The type VI secretion system (T6SS) is a widespread protein export apparatus found in Gram-negative bacteria. T6SSs mediate bacterial antagonism by facilitating the injection of toxic effector proteins into competing bacterial cells in a contact-dependent manner. Here, we present the structures of the T6SS effector RhsA from Pseudomonas protegens and its cognate T6SS spike protein, VgrG1, at 3.3 Å resolution. The rhsA operon contains genes encoding its cognate VgrG spike and Eag chaperone proteins, both of which are required for the delivery of this effector into susceptible competitors.

To investigate how RhsA is mounted onto VgrG1 we set out to determine the structure of the secretion competent pre-firing complex (PFC) comprising VgrG1 in complex with full-length RhsA and EagR1. Unfortunately, this conformational heterogeneity prevented us from obtaining a high-resolution 3D reconstruction of the entire complex. Instead, we applied C3 symmetry during processing to determine the three-dimensional structure of P. protegens VgrG1. In applying this symmetry operator, the RhsA and EagR1 components of the complex, which do not adopt this symmetry, are averaged out during image processing. The cryo-EM map of VgrG1 reached a resolution of 3.3 Å and allowed us to build almost the complete atomic model of the protein comprising residues 8–643. As expected, given its high sequence homology, the structure of VgrG1 from P. protegens is nearly identical (71% sequence identity, 81% sequence similarity) to our previously determined VgrG1 structure from P. aeruginosa (r.m.s.d of 1.035 between 544 pruned Cα atoms; r.m.s.d of 1.428 across the complete structure, S9B and S9C Fig) even though their respective effectors, RhsA and Tse6, bear no sequence or structural similarity to one another beyond their N-terminal prePAAR and PAAR domains. Intriguingly, we identified two spherical densities in the center of the β-sheet prism of the VgrG1 trimer. Based on the exclusive clustering of positively charged residues around this density and its overall size, we hypothesize that it corresponds to either a phosphate or sulfate anion, which probably helps to stabilize the core of VgrG1 given that in the absence of this anion, the presence of positively charged residues in the core of the protein would be energetically unfavorable.

>MLFQQSTRLAQVNCPLGPDVLLLKSLGGGEELGRLFDYQLQLASSDANIDLNQLLGKPMGLSVQLDGGGQRYFHGIVARCSQNIDTGQFASYEVTLRPWLWLLSRTSDCRIFQNLSIPQIIKQVFRDLGFSDFEDALSRPYREWEYCVQYRETSFDFVSRLMEQEGIYYFFRHEKDRHVVVLADAYGAHSSVPGYASVPYYPRDEQQRERDHMFDWHLAQEVQPGSLELNDYDFQRPSARIDVRSAMPRPHSAGDYPLYDYPGTYVQSSDGEHYAQTRIEALQSLHERIELSGNARGLGVGNLFSLTGFSRQDQNREYLIVSIRYYLVQESLESGAGGGSAQFESHLTCIDAQQSFRPLATTHKPMVQGPQTARVVGPAGEEIWTDQYGRVKVHFHWDRHDQSNENSSCWIRVSQAWAGKNWGSMQIPRIGQEVIVSFLEGDPDRPIITGRVYNAEQTVPYDLPANATQSGMKSRSSKGGSPANFNEIRMEDKKGAEQLYIHAERNQDIVVEVNESHSVGNNRNKSIGHDEYVTIGNKRTRIVQHVDELRVGEKKLDSVGQSYVIEVGERLRLVCGASILELNASGQINLCGVNISVHASADAQINTGGVLHLNNGGGPGTTTEGQGVQGAISAKAKAPFSAPKG[3x]>MNAYYIQDRLEAQSWARHYQQLAREEKEAELADDMEKGIPQHLFESLCIDHLQRHGASKKSITRAFDDDVEFQERMAEHIRYMVETIAHHQVDIDSEV[2x];> GMSDVAETLDPLRLPLQGERLIEASAGTGKTFTIAALYLRLLLGLGGSAAFPRPLTVEELLVVTFTEAATAELRGRIRSNIHELRIACLRETTDNPLYERLLEEIDDKAQAAQWLLLAERQMDEAAVFTIHGFCQRMLNLNAFESGMLFEQQLIEDESLLRYQACADFWRRHCYPLPREIAQVVFETWKGPQALLRDINRYLQGEAPVIKAPPPDDETLASRHAQIVARIDTVKQQWRDAVGELDALIESSGIDRRKFNRSNQAKWIDKISAWAEEETNSYQLPESLEKFSQRFLEDRTKAGGETPRHPLFEAIDQLLAEPLSIRDLVITRALAEIRETVAREKRRRGELGFDDMLSRLDSALRSESGEVLAAAIRTRFPVAMIDEFQDTDPQQYRIFRRIWHHQPETALLLIGDPKQAIYAFRGADIFTYMKARSEVHAHYTLDTNWRSAPGMVNSVNKLFSQTDDAFMFREIPFIPVKSAGKNQALRFVFKGETQPAMKMWLMEGESCGVGDYQSTMAQVCAAQIRDWLQAGQRGEALLMNGDDARPVRASDISVLVRSRQEAAQVRDALTLLEIPSVYLSNRDSVFETLEAQEMLWLLQAVMTPERENTLRSALATSMMGLNALDIETLNNDEHAWDVVVEEFDGYRQIWRKRGVMPMLRALMSARNIAENLLATAGGERRLTDILHISELLQEAGTQLESEHALVRWLSQHILEPDSNASSQQMRLESDKHLVQIVTIHKSKGLEYPLVWLPFITNFRVQEQAFYHDRHSFEAVLDLNAAPESVDLAEAERLAEDLRLLYVALTRSVWHCSLGVAPLVRRRGDKKGDTDVHQSALGRLLQKGEPQDAAGLRTCIEALCDDDIAWQTAQTGDNQPWQVNDVSTAELNAKTLQRLPGDNWRVTSYSGLQQRGHGIAQDLMPRLDVDAAGVASVVEEPTLTPHQFPRGASPGTFLHSLFEDLDFTQPVDPNWVREKLELGGFESQWEPVLTEWITAVLQAPLNETGVSLSQLSARNKQVEMEFYLPISEPLIASQLDTLIRQFDPLSAGCPPLEFMQVRGMLKGFIDLVFRHEGRYYLLDYKSNWLGEDSSAYTQQAMAAAMQAHRYDLQYQLYTLALHRYLRHRIADYDYEHHFGGVIYLFLRGVDKEHPQQGIYTTRPNAGLIALMDEMFAGMTLEEA;> MLRVYHSNRLDVLEALMEFIVERERLDDPFEPEMILVQSTGMAQWLQMTLSQKFGIAANIDFPLPASFIWDMFVRVLPEIPKESAFNKQSMSWKLMTLLPQLLEREDFTLLRHYLTDDSDKRKLFQLSSKAADLFDQYLVYRPDWLAQWETGHLVEGLGEAQAWQAPLWKALVEYTHQLGQPRWHRANLYQRFIETLESATTCPPGLPSRVFICGISALPPVYLQALQALGKHIEIHLLFTNPCRYYWGDIKDPAYLAKLLTRQRRHSFEDRELPLFRDSENAGQLFNSDGEQDVGNPLLASWGKLGRDYIYLLSDLESSQELDAFVDVTPDNLLHNIQSDILELENRAVAGVNIEEFSRSDNKRPLDPLDSSITFHVCHSPQREVEVLHDRLLAMLEEDPTLTPRDIIVMVADIDSYSPFIQAVFGSAPADRYLPYAISDRRARQSHPVLEAFISLLSLPDSRFVSEDVLALLDVPVLAARFDITEEGLRYLRQWVNESGIRWGIDDDNVRELELPATGQHTWRFGLTRMLLGYAMESAQGEWQSVLPYDESSGLIAELVGHLASLLMQLNIWRRGLAQERPLEEWLPVCRDMLNAFFLPDAETEAAMTLIEQQWQAIIAEGLGAQYGDAVPLSLLRDELAQRLDQERISQRFLAGPVNICTLMPMRSIPFKVVCLLGMNDGVYPRQLAPLGFDLMSQKPKRGDRSRRDDDRYLFLEALISAQQKLYISYIGRSIQDNSERFPSVLVQELIDYIGQSHYLPGDEALNCDESEARVKAHLTCLHTRMPFDPQNYQPGERQSYAREWLPAASQAGKAHSEFVQPLPFTLPETVPLETLQRFWAHPVRAFFQMRLQVNFRTEDSEIPDTEPFILEGLSRYQINQQLLNALVEQDDAERLFRRFRAAGDLPYGAFGEIFWETQCQEMQQLADRVIACRQPGQSMEIDLACNGVQITGWLPQVQPDGLLRWRPSLLSVAQGMQLWLEHLVYCASGGNGESRLFLRKDGEWRFPPLAAEQALHYLSQLIEGYREGMSAPLLVLPESGGAWLKTCYDAQNDAMLDDDSTLQKARTKFLQAYEGNMMVRGEGDDIWYQRLWRQLTPETMEAIVEQSQRFLLPLFRFNQS;> MGKLQKQLLEAVEHKQLRPLDVQFALTVAGDEHPAVTLAAALLSHDAGEGHVCLPLSRLENNEASHPLLATCVSEIGELQNWEECLLASQAVSRGDEPTPMILCGDRLYLNRMWCNERTVARFFNEVNHAIEVDEALLAQTLDKLFPVSDEINWQKVAAAVALTRRISVISGGPGTGKTTTVAKLLAALIQMADGERCRIRLAAPTGKAAARLTESLGKALRQLPLTDEQKKRIPEDASTLHRLLGAQPGSQRLRHHAGNPLHLDVLVVDEASMIDLPMMSRLIDALPDHARVIFLGDRDQLASVEAGAVLGDICAYANAGFTAERARQLSRLTGTHVPAGTGTEAASLRDSLCLLQKSYRFGSDSGIGQLAAAINRGDKTAVKTVFQQDFTDIEKRLLQSGEDYIAMLEEALAGYGRYLDLLQARAEPDLIIQAFNEYQLLCALREGPFGVAGLNERIEQFMQQKRKIHRHPHSRWYEGRPVMIARNDSALGLFNGDIGIALDRGQGTRVWFAMPDGNIKSVQPSRLPEHETTWAMTVHKSQGSEFDHAALILPSQRTPVVTRELVYTAVTRARRRLSLYADERILSAAIATRTERRSGLAALFSSRE

In bacterial cells, the related AddAB and RecBCD enzymes are helicase-nuclease complexes responsible for initiating homologous recombination from double-stranded DNA breaks (DSBs). This activity underpins many key DNA transactions including DSB repair, phage restriction, and conjugal or transductional recombination. For example, phage λ Gam is a potent inhibitor of the Escherichia coli RecBCD complex that helps to protect the phage DNA from degradation. In this work, we present the structure of Gam bound to RecBCD unveiling an inhibition mechanism based on protein mimicry of a DSB.

Previous work has shown that GamS inhibits RecBCD by competing with DNA binding. The structure we present here, of the GamS dimer complexed with RecBCD, was determined by cryo-electron microscopy at 3.8 Å resolution (Figure 1—source data 1, Figure 1—figure supplements 1 and 2). It reveals that the GamS protein does indeed act as a steric block to the binding of DNA. The interaction with the duplex DNA-binding ‘arm’ of the RecB subunit is extensive and overlaps completely with that of the duplex DNA binding site. Furthermore, one of the long N-terminal helical extensions of GamS inserts deeply into RecBCD. It occupies a channel that normally accommodates the nascent 3’-ssDNA tail bound to the RecB helicase subunit, increasing the extent of the steric block. Although the structure of the RecBCD complex is closest to that of the initiation complex it responds to the binding of Gam by small changes in conformation. The 2B and C-terminal domains of the RecC subunit together with the 2B domain of RecB move as a unit away from the RecB helicase domains. The crystal structure of the GamS protein alone revealed a pattern of negative charges on the surface that mimicked a DNA duplex, suggesting that molecular mimicry might be involved in binding. Consistent with this idea, a series of acidic side chains on Gam are located in positions equivalent to the phosphates of the DNA backbone and interact with many of the same residues on the RecBCD surface. Instead, the main component of the interaction is simply a steric block; the helix makes a snug fit in the channel involving many more contacts than the equivalent contacts with ssDNA.>MRRVLVAGNWKMHKTPSEARVWFAELKRLLPPLQSEAAVLPAFPILPVAKEVLAETQVGYGAQDVSAHKEGAYTGEVSARMLSDLGCRYAIVGHSERRRYHGETDALVAEKAKRLLEEGITPILCVGEPLEVREKGEAVPYTLRQLRGSLEGVEPPGPEALVIAYEPVWAIGTGKNATPEDAEAMHQAIRKALSERYGEAFASRVRILYGGSVNPKNFADLLSMPNVD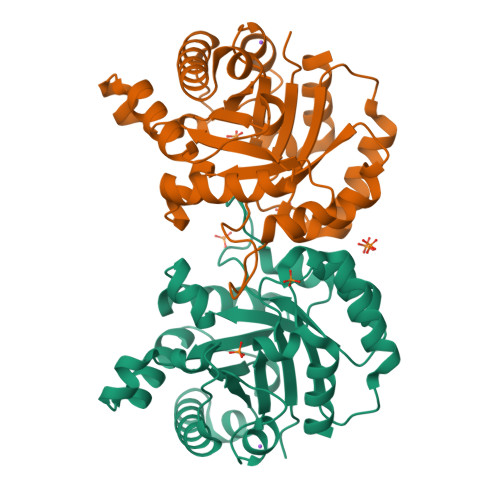GGLVGGASLELESFLALLRIAG[2x]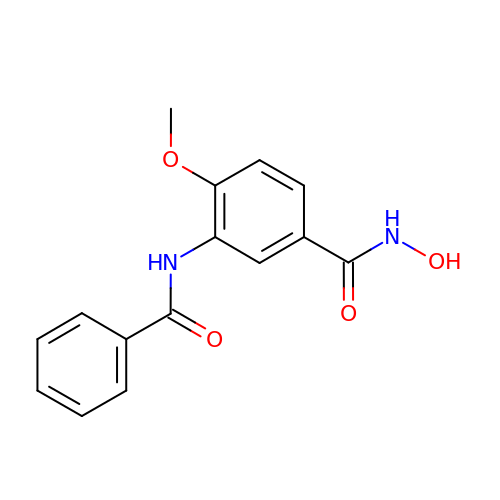3-benzamido-4-methoxy-~{N}-oxidanyl-benzamide | C15 H14 N2 O4 | XJRKOVTYPFIMNR-UHFFFAOYSA-N> GAKESEQKVTIDSAKHEKHTKDKEENNSANTVFFDKINDLLVASVKEFEGTVGISYLDLETGEQRSVNGQHEFYTASTIKVPLTMLVADTVASGQK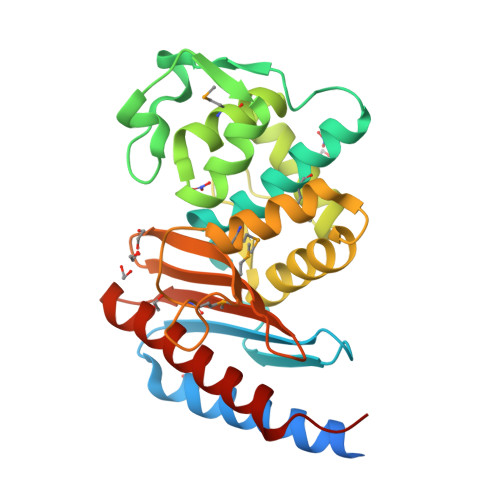KWTDLIPYNAEEDYEEGTGIIAYNIQPEYPLKTLQEYAITYSDNIAKNMLYDTLGGDAKAKREMYQRYLHKTPSIEEPQFSSEDALVILQKLYTEKATKPDYQAIYDSMKQSVFHERMETPTTQGKVAHKIGSYDEFIHDMGILETPHPFALAIFTKGPDNAKSAAFIASVTDKLWQLQVSEYPNQ>[4x]MSILKIHAREIFDSRGNPTVEVDLFTSKGLFRAAVPSGASTGIYEALELRDNDKTRYMGKGVSKAVEHINKTIAPALVSKKLNVTEQEKIDKLMIEMDGTENKSKFGANAILGVSLAVCKAGAVEKGVPLYRHIADLAGNSEVILPVPAFNVINGGSHAGNKLAMQEFMILPVGAANFREAMRIGAEVYHNLKNVIKEKYGKDATNVGDEGGFAPNILENKEGLE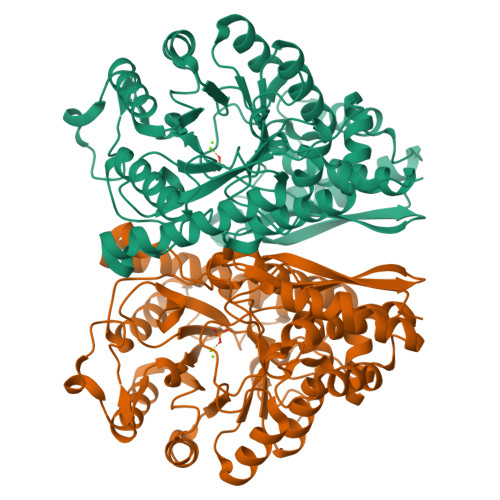LLKTAIGKAGYTDKVVIGMDVAASEFFRSGKYDLDFKSPDDPSRYISPDQLADLYKSFIKDYPVVSIEDPFDQDDWGAWQKFTASAGIQVVGDDLTVTNPKRIAKAVNEKSCNCLLLKVNQIGSVTESLQACKLAQANGWGVMVSHRSGETEDTFIADLVVGLCTGQIKTGAPCRSERLAKYNQLLRIEEELGSKAKFAGRNFRNPLAK>AQVINTFDGVADYLQTYHKLPDNYITKSEAQALGWVASKGNLADVAPGKSIGGDIFSNREGKLPGKSGRTWREADINYTSGFRNSDRILYSSDWLIYKTTDHYQTFTKIR[3x];>KKAVINGEQIRSISDLHQTLKKELALPEYYGENLDALWDALTGWVEYPLVLEWRQFEQSKQLTENGAESVLQVF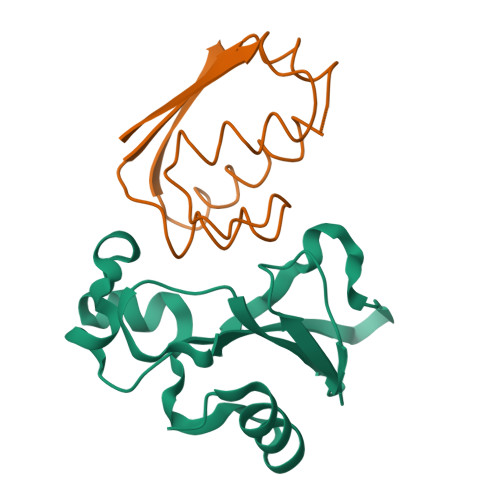REAKAEGADITIILS[3x]> SNAPVTELTRLKEYMEDQIAKAKESSSLTAQLKFLENAHTEHFVKMGSLT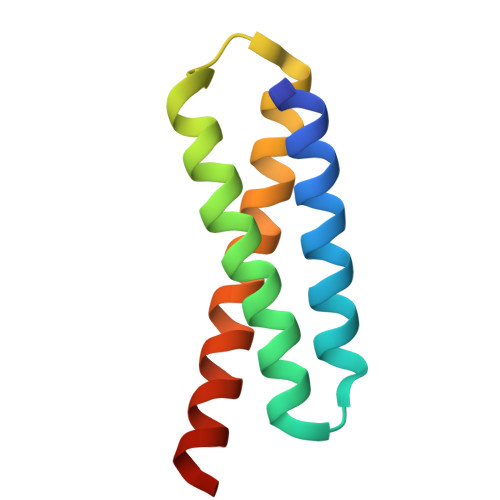TIYKGGSEVVDRLKIEIRSLYEEMLELKDKCRDQIQQYETS Several lines of evidence implicate the human activating signal co-integrator complex (ASCC) in AlkBH3-mediated DNA repair. ASCC3 is the largest subunit of ASCC and was characterized as a DNA helicase that unwinds DNA by translocating on one strand in 3’-to-5’ direction. ASCC and alkylated nucleotides co-localize at nuclear foci upon alkylation damage stress, dependent on a coupling of ubiquitin conjugation to ER degradation (CUE) domain in ASCC2, which links DNA alkylation damage repair to upstream ubiquitin signaling via the RING finger protein 113A9. As a member of the Ski2-like family of superfamily (SF) 2 nucleic acid helicases, ASCC3 shows striking resemblance to the pre-mRNA splicing factor Brr2 (sequence identity of 41/33% between human ASCC3 and human/yeast Brr2), an ATP-dependent RNA helicase that is essential for spliceosome activation, catalysis and disassembly.

Here, we mapped precise interacting regions of the two largest ASCC subunits, ASCC2 and ASCC3, and determined a crystal structure of an ASCC2–ASCC3 complex comprising these portions. Guided by the structure, we delineated segments and residues that are critical for the ASCC2–ASCC3 interaction, which include a large number of residues that are altered by somatic cancer mutations. The importance of regions for the interaction scales with the degree of their evolutionary conservation. Moreover, we observed that a large number of ASCC2 and ASCC3 residue substitutions encoded by somatic mutations in cancers map to ASCC2–ASCC3 interface regions and that selected, cancer-related residue substitutions in ASCC3 lead to reduced ASCC2–ASCC3 affinity. Our structural analysis revealed that ASCC3 and Brr2 share at least some structural organization in their NTRs as well. Both contain a plug/plug-like domain close to their N-termini (residues 59–142 in human ASCC3, 113–192 in yeast Brr2, 107–180 in human Brr2). Based on our crystal structure, regions neighboring the ASCC3 plug-like domain are expected to be guided away from the ASCC3 helicase region when bound to ASCC2, however, ASCC2 did not alleviate ASCC3 auto-inhibition. ASCC3 auto-inhibition may, therefore, be predominantly mediated via the plug-like domain, which remains accessible in complex with ASCC2, occupying a position on the helicase region where it competes with DNA substrate loading. Correlation of the evolutionary conservation of ASCC2–ASCC3 interfaces and the contributions of these regions to a stable interaction underscore the functional importance of the complex we structurally analyzed. Based on these observations and previous insights into the role of ASCC components in DNA alkylation damage repair, we suggest that reduced ASCC2–ASCC3 affinity might contribute to malignant transformation.

> GAEFMALPRLTGALRSFSNVTKQDNYNEEVADLKIKRSKLHEQVLDLGLTWKKIIKFLNEKLEKSKMQSINEDLKDILHAAKQIVGTDNGREAIESGAAFLFMTFHLKDSVGHKETKAIKQMFGPFPSSSATAACNATNRIISHFSQDDLTALVQMTEKEHGDRVFFGKNLAFSFDMHDLDHFDELPINGETQKTISLDYKKFLNEHLQEA;> GAMAMPALPLDQLQITHKDPKTGKLRTSPALHPEQKADRYFVLYKPPPKDNIPALVEEYLERATFVANDLDWLLALPHDKFWCQVIFDETLQKCLDSYLRYVPRKFDEGVASAPEVVDMQKRLHRSVFLTFLRMSTHKESKDHFISPSAFGEILYNNFLFDIPKILDLCVLFGKGNSPLLQKMIGNIFTQQPSYYSDLDETLPTILQVFSNILQHCGLQGDGANTTPQKLEERGRLTPSDMPLLELKDIVLYLCDTCTTLWAFLDIFPLACQTFQKHDFCYRLASFYEAAIPEMESAIKKRRLEDSKLLGDLWQRLSHSRKKLMEIFHIILNQICLLPILESSCDNIQGFIEEFLQIFSSLLQEKRFLRDYDALFPVAEDISLLQQASSVLDETRTAYILQAVESAWEGVDRRKATDAKDPSVIEEPNGEPNGVTVTA> DINGGGATLPQKLYLTPDVLTAGFAPYIGVGSGKGKIAFLENKYNQFGTDTTKNVHWAGSDSKLTATELATYAADKEPGWGKLIQVPSVATSVAIPFRKAGANAVDLSVKELCGVFSGRIADWSGITGAGRSGPIQVVYRAESSGTTELFTRFLNAKCTTEPGTFAVTTTFANSYSLGLTPLAGAVAATGSDGVMAALNDTTVAEGRITYISPDFAAPTLAGLDDATKVA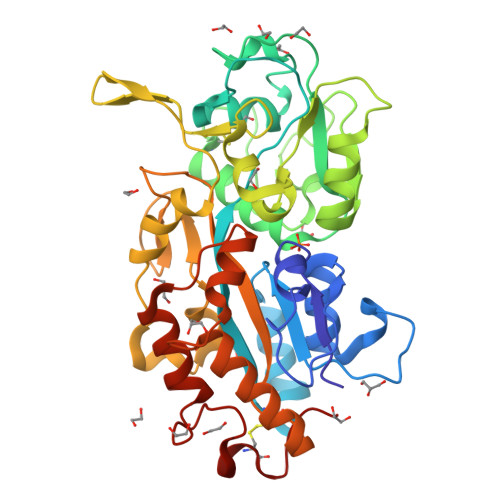RVGKGVVNGVAVEGKSPAAANVSAAISVVPLPAAADRGNPDVWVPVFGATTGGGVVAYPDSGYPILGFTNLIFSQCYANATQTGQVRDFFTKHYGTSANNDAAIEANAFVPLPSNWKAAVRASFLTASNALSIGNTNVCNGKGRPQ>SNAMSQEAFENKLYANLE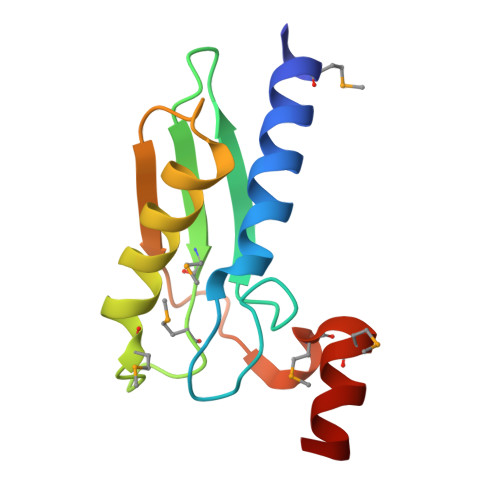AVIDPELGVDIVNLGLVYDVTADENNNAVITMTMTSIGCPMAGQIVSDVKKVLSTNVPEVNEIEVNVVWNPPWSKERMSRMAKIALGIRD[6x]> MGHHHHHHGSENLYFQGSGQRWELALGRFWDYLRWVQTLSEQVQEEL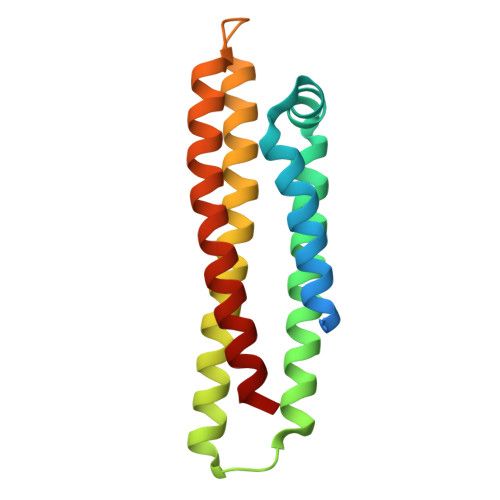LSSQVETKLNKLMQRTMEELKAYKSELEEQLTPVAEETRARLSKELQAAQARLGADMEDVCGRLVQYRGEVQAMLGQSTEELRVRLATHLNKLRQRLLEDADDLQKRLAVYQ>MSESPMFAANGMPKVNQGAEEDVRILGYDPLASPALLQVQIPATPTSLETAKRGRREAIDIITGKDDRVLVIVGPCSIHDLEAAQEYALRLKKLSDELKGDLSIIMRAYLEKPRTTVGWKGLINDPDVNNTFNINKGLQSARQLFVNLTNIGLPIGSEMLDTISPQYLADLVSFGAIGARTTESQLHRELASGLSFPVGFKNGTDGTLNVAVDACQAAAHSHHFMSVTKHGVAAITTTKGNEHCFVILRGGKKGTNYDAKSVAE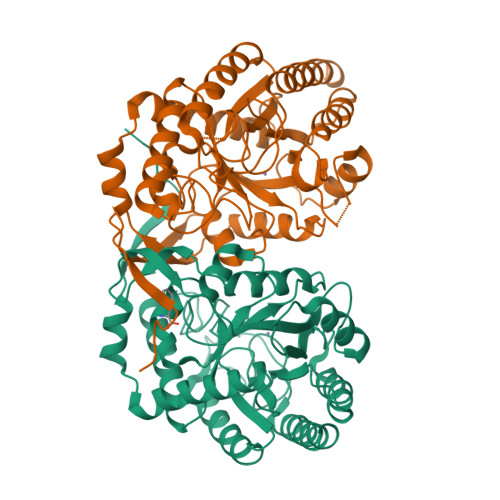AKAQLPAGSNGLMIDYSHGNSNKDFRNQPKVNDVVCEQIANGENAITGVMIESNINEGNQGIPAEGKAGLKYGVSITDACIGWETTEDVLRKLAAAVRQRREVNKK[8x]> MSLTNDERILSWNETPSKPRYTPPPGAIDAHCHVFGPMAQFPFSPKAKYLPRDAGPDMLFALRDHLGFARNVIVQASCHGTDNAATLDAIARAQGKARGIAVVDPAIDEAELAALHEGGMRGIRFNFLKRLVDDAPKDKFLEVAGRLPAGWHVVIYFEADILEELRPFMDAIPVPIVIDHM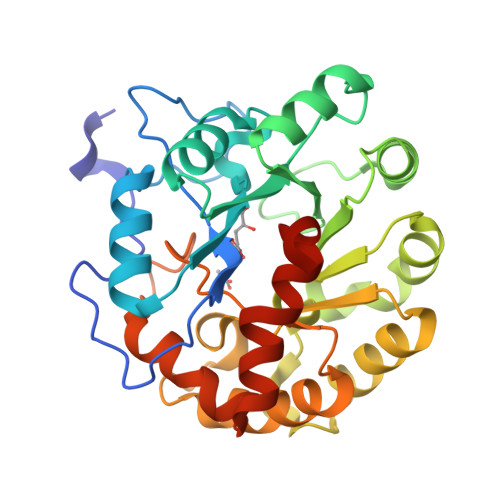GRPDVRQGPDGADMKAFRRLLDSREDIWFKATCPDRLDPAGPPWDDFARSVAPLVADYADRVIWGTAWPHPNMQDAIPDDGLVVDMIPRIAPTPELQHKMLVTNPMRLYWSEEMEGHHHHHH One especially common junction element is the kink-turn (k-turn). k-turns are elements in double-stranded RNA that introduce a tight kink into the helical axis, with an included angle close to 50°. A standard k-turn comprises a three-nucleotide bulge followed by successive G•A and A•G trans G(sugar edge)•A(Hoogsteen edge) basepairs. k-turns are commonly-occurring motifs that introduce sharp kinks into duplex RNA, thereby facilitating tertiary contacts. Both the folding and conformation of k-turns are determined by their local sequence. k-turns fall into two conformational classes, called N3 and N1, that differ in the pattern of hydrogen bonding in the core. We show here that this is determined by the basepair adjacent to the critical G•A pairs.

We therefore decided to extend the study with a systematic structural analysis of HmKt-7 as a function of the 3b,3n sequence. This was performed in the constant environment of the SAM-I riboswitch, modified by replacing its natural k-turn by HmKt-7 with different 3b,3n sequences. In this way we could observe the effect of changing the 3b,3n sequence alone in an otherwise completely unchanged RNA molecule. There are also three examples of 3b,3n = U•G; in this case each adopts the N1 conformation. Interestingly, each 3b,3n = U•G k-turn exists in a different environment, in a riboswitch (cobalamine), ribosome (Thermus thermophilus Kt-7 (25)), or bound by the ScL30e protein. Yet the correlation between 3b,3n = U•G and the N1 conformation holds good for each. Where the modified HmKt-7 elements have the same 3b,3n sequence as a different k-turn, they adopt the same conformation as that structure. Altogether seven of the new structures are in the N1 conformation, and clearly simply changing the 3b,3n sequence alone is sufficient to induce the structure of Kt-7 to change within the riboswitch environment. The N3 group contain a preponderance of 3b,3n = A•G and U•U pairs, and the N1 group comprise mainly 3b,3n = U•G, C•A and C•C pairs. A marked preference (92.06%) for 3b,3n = U•G is clear.

> GGCUUAUCAAGAGAGGGGGAGCGACUGGCGCGAAGAUCCCCGGCAACCAGAAAUGGUGCCAAUUCCUGCAGCGGAAACGUUGAAAGAUGAGCCG Nylon hydrolase (NylC) is one of the three enzymes responsible for the endo-type degradation of the by-products of nylon-6 manufacture (cyclic and linear oligomers of 6-aminohexanoate (Ahx) with a degree of polymerization greater than three) and various aliphatic nylons (e.g., nylon-6 and nylon-66). However, the post-translational autocleavage of the nascent polypeptide between Asn266 and Thr267 generates an active enzyme with an α subunit (27 kDa) and a β subunit (9 kDa). Based on the X-ray-crystallographic structure of NylCA, we reported that four αβ heterodimers (molecules A-D) form a doughnut-shaped quaternary structure. In addition, we proposed that the nucleophilic N-terminal residue Thr267 in the β subunit functions as a catalytic residue for either autocleavage (from precursor to active enzyme) or substrate hydrolysis.

Three amino acid residues corresponding to the substitutions D122G, H130Y, and D36A (increasing the protein stability of NylCp2) and one amino acid residue corresponding to the substitution L137A (decreasing the protein stability) were located at the A/D interface, and the glutamate residue corresponding to the substitution E263Q was found at the A/B interface. In the G122Y130A36Q263 mutant, the acidic amino acid residue Glu263 was replaced with a neutral Gln, suggesting that the alterations in the electrostatic environment induced by the E263Q mutation contributed to improving the subunit interactions. We confirmed that the E263Q substitution in G122Y130A36 (Tm = 84 °C) increased thermostability by 4 °C9. The rmsd of the main-chain atoms between NylCp2 and NylCA and between NylCp2 and NylCp2-G122Y130A36Q263 was generally less than 1 Å, but loop 1 (positions 15–34), loop 2 (positions 88–93), loop 3 (positions 125–133), α3 (positions 246–257), loop 5 (positions 258–269), and loop 7 (positions 319–333) displayed significant structural differences. It should be noted that α1 and its adjacent loop 3 regions showed the largest structural difference between NylCA and NylCp2, whereas a difference of less than 2 Å was found between NylCA and NylCp2-G122Y130A36Q263. Wild-type NylCK and the most thermostable mutant, NylCp2-G122Y130A36Q263 (Tm = 88 °C), should exist mainly as a tetramer of αβ-heterodimers (MAV = 151,384 and 130,895, respectively). The absence of a dimer molecule suggested that the equilibrium of reactions 1 and 2 were optimized to yield tetramers as the major product, leaving monomers as a minor population.

>MNTTPVHALTDIDGGIAVDPAPRLAGPPVFGGPGNAAFDLAPVRSTGREMLRFDFPGVSIGAAHYEEGPTGATVIHIPAGARTAVDARGGAVGLSGGYDFNHAICLAGGAGYGLEAGAGVSGALLERLEYRTGFAELQLVSSAVIYDFSARSTAVYPDKALGRAALEFAVPGEFPQGRAGAGMSASAGKVDWDRTEITGQGAAFRRLGDVRILAVVVPNPVGVIVDRAGTVVRGNYDAQTGVRRHPVFDYQEAFAEQVPPVTQAGNTTISAIVTNVRMSPVELNQFAKQVHSSMHRGIQPFHTDMDGDTLFAVTTDEIDLPTTPGSSRGRLSVNATALGAIASEVMWDAVLEAGK[2x]>GIDPFTKTSLYESTLKNQTDLLKVTQSTVEDFRSTNQSFTRALEKDIANLPYQSLITEENIINNVGPILKYYRHSINALNVYLGLNNGKVLLSQKSNDAKMPELRDDLDIKTKDWYQEALKTNDIFVTPAYLD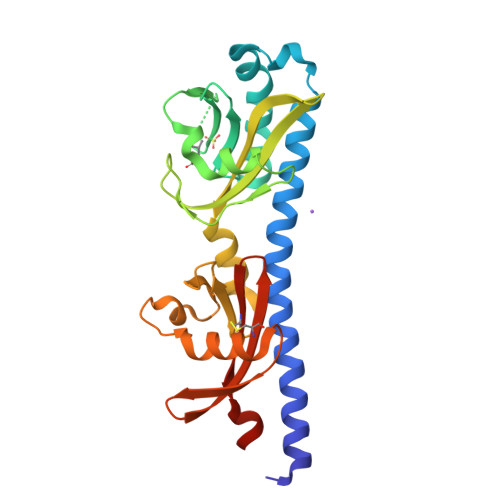TVLKQYVITYSKAIYKDGKIIGVLGVDIPSEDLQNLVAKTPGNTFLFDQKNKIFAATNKELLNPSIDHSPVLNAYKLNGDNNFFSYKLNNEERLGACTKVFAYTACITESADIINKPIYKA[2x]> GSHMLRLSAPGQLDDDLCLLGDVQVPVFLLRLGEASWALVEGGISRDAELVWADLCRWVADPSQVHYWLITHKHYDHCGLLPYLCPRLPNVQVLASERTCQAWKSESAVRVVERLNRQLLRAEQRLPEACAWDALPVRAVADGEWLELGPRHRLQVIEAHGHSDDHVVFYDVRRRRLFCGDALGWFDEAEGVWRPLVFDDMEAYLESLERLQRLPTLLQLIPGHGGLLRGRLAADGAESAYTECLRLCRRLLWRQSMGESLDELSEELHRAWGGQSVDFLPGALHLGSMRRMLEILSRQALPLD

PqsE has two biochemical activities, a protein–protein interaction with RhlR, which increases RhlR transcriptional activity at target promoters, and an esterase activity. Curiously, RhlR function additionally depends on the metallo-β-hydrolase enzyme PqsE, encoded as the final gene in the pqsABCDE biosynthetic operon. With respect to RhlR, PqsE is required to form a protein–protein interaction that enhances the affinity of RhlR for target promoters. The effects of the PqsE E182W and PqsE NI substitutions on pyocyanin production are not through impairment of PqsE catalytic function, as the catalytically inactive variant, PqsE(D73A), remains fully capable of interacting with RhlR and driving pyocyanin production. These results indicate that PqsE has two independent functions, catalysis and interaction with RhlR, and it is interaction with RhlR, not catalysis, that is required for virulence. Moreover, the RhlR–PqsE interaction is essential for P. aeruginosa virulence phenotypes, and therefore, of interest as a focus for antibiotic development.

To test whether repositioning of the PqsE E280 residue underpinned the inhibitor mimetic characteristics of the PqsE(E182W) protein, we engineered the E280A substitution into PqsE(E182W) to make PqsE(E182W/E280A). We determined the crystal structure of PqsE(E182W/E280A) revealing further changes in the PqsE active site. In this case, the presence of an alanine at residue 280 eliminated interaction with the iron atoms, and the loop consisting of residues D275-L281 was disordered. The remainder of the loop was ordered and its structure reverted to a conformation that was more native-like than in PqsE(E182W). Consequently, the removal of the glutamate–Fe interaction via the E280A substitution apparently unblocked the active site of PqsE, partially restoring WT activity. Indeed, whereas PqsE(E182W) exhibits reduced binding affinity for the active site fluorescent probe, BB562, PqsE(E182W/E280A) displays WT binding affinity for the probe. The catalytic function of the PqsE(E182W/E280A) variant was greatly improved by the “unblocking” of the active site (34% compared to WT PqsE). Consistent with the repositioning of E280 into the PqsE active site contributing to the increased stability of the PqsE(E182W) protein relative to WT PqsE, introduction of the E280A substitution reduced the Tm of the PqsE(E182W/E280A) protein to nearly that of WT PqsE. Nonetheless, the PqsE(E182W/E280A) variant remains incapable of enhancing RhlR transcription factor activity in an Escherichia coli reporter assay and it does not drive pyocyanin production in P. aeruginosa PA14 (respectively). Analysis of the PqsE(E182W/E280A) structure, and the surprisingly modest conformational changes that are apparent compared to the structures of WT PqsE and PqsE(E182W), suggest that the structural integrity of the G270-L281 loop is essential for PqsE to interact with RhlR.> SEISRQEFQRRRQALVEQMQPGSAALIFAAPEVTRSADSEYPYRQNSDFWYFTGFNEPEAVLVLIKSDDTHNHSVLFNRVRDLTAEIWFGRRLGQDAAPEKLGVDRALAFSEINQQLYQLLNGLDVVYHAQGEYAYADVIVNSALEKLRKGSRQNLTAPATMIDWRPVVHEMRLFKSPEEIAVLRRA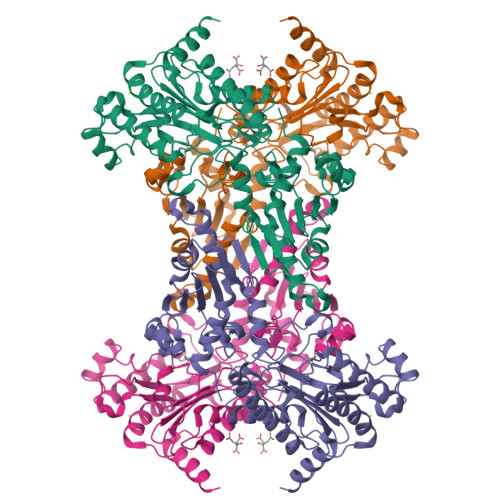GEITAMAHTRAMEKCRPGMFEYHLEGEIHHEFNRHGARYPSYNTIVGSGENGCILHYTENECEMRDGDLVLIAAGCEYKGYAGDITRTFPVNGKFTQAQREIYDIVLESLETSLRLYRPGTSILEVTGEVVRIMVSGLVKLGILKGDVDELIAQNAHRPFFMHGLSHWLGLDVHDVGVYGQDRSRILEPGMVLTVEPGLYIAPDAEVPEQYRGIGIRIEDDIVITETGNENLTASVVKKPEEIEALMVAARKQ>SQLLNYIDGNFVTSASSFANINPVNGKLISDVFEADAKQVNEAVVAAQNALKGPWGKLSVQDRAALIHKIADGIQARFEEFVAAEVADTGRPVHQARTLDIPRAIANFRTFADLAKTSHTDLFEMSTSDGSGALNYTVRKPLGVIGVISPWNLPLLLFTWKVAPALACGNTVVAKPSEESPSSATLLAEVMHDAGVPPGVFNLIHGFGKDSAGEFLTQHPGISALTFTGESKTGSTIMKAVADGVKEVSFALGGKNAAVVFADADLDAAIEGVLRSSFTNSGQVCLCSERVYVHRSIFDEFVSGLKVEAERLVVGYPDQDGVNMGPLISHGHRDKVLSYYRLAVDEGATVVTGGGVPKFNDERDQGAYVQPTIWTGLSDKARCVTEEIFGPVCHISPFDDEDEVINRVNDSNYGLACAIWTTNLSRAHRVSRQIHVGLVWVNTWYLRDLRTPFGGVKLSGLGREGGRFSMDFYSDIANICIKI[4x]

One enzyme in particular, 2-aminomuconate-6-semialdehyde dehydrogenase (AMSDH), is responsible for oxidizing the unstable metabolic intermediate 2-aminomuconate-6-semialdehyde (2-AMS) to 2-aminomuconate (2-AM). On the basis of sequence alignment, AMSDH is a member of the hydroxymuconic-semialdehyde dehydrogenase (HMSDH) family under the aldehyde dehydrogenase (ALDH) superfamily. The complete AMSDH model includes four polypeptides per asymmetric unit describing one homotetramer. Each monomer of AMSDH contains three domains: a subunit interaction domain, a catalytic domain and an NAD+ binding domain.

The nature of the absorbing species at 422 nm was further investigated by soaking co-crystallized E268A-NAD+ crystals in mother liquor containing 2-HMS. When E268A-NAD+ crystals are soaked with 2-HMS for 40 min or less, their single-crystal electronic absorption spectra show an absorbance maximum at 422 nm, as was observed in the solution-state titration and the stopped-flow assays. The structure of E268A-NAD+ soaked with 2-HMS for 30 min before flash cooling was solved and refined to 2.15 Å resolution. In this structure, a continuous electron density between Cys302-SG and 2-HMS-C6 is observed, similar to the thioacyl intermediate observed in the wild-type enzyme. However, in contrast to the thioacyl intermediate, the density around C6 is less flat, indicating an sp3- rather than sp2-hybridized carbon. The angle between the plane of the carbon backbone of the substrate and the formerly aldehydic oxygen is 55±9°, compared with the angle of the wild-type thioacyl intermediate at 26±4°. More importantly, the C6 of 2-HMS and the C4N of NAD+ are very close (2.4–2.8 Å), making it unlikely that the hydride has been transferred from the substrate. Taken together, these data allow us to assign this intermediate to a thiohemiacetal enzyme adduct. However, in this work, the E268A mutant is shown to accumulate the preceding thiohemiacetal intermediate both in crystal and in solution. This finding suggests an additional catalytic role for this residue: rotation of Glu268 towards the active site facilitates the hydride transfer from the tetrahedral thiohemiacetal adduct to NAD+.isothiocyanate | C H N 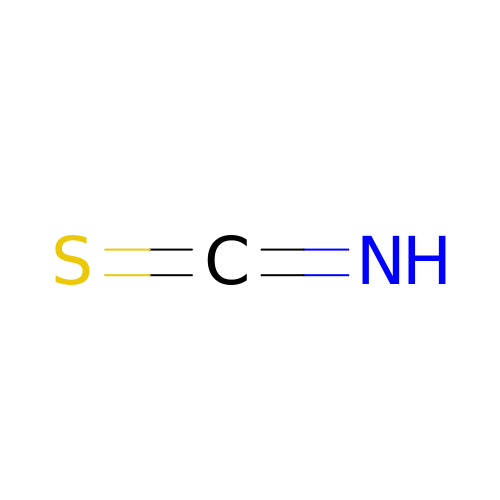S | GRHBQAYDJPGGLF-UHFFFAOYSA-N>[2x]DTLESIDNCAVGCPTGGSSNVSIVRHAYTLNNNSTTKFANW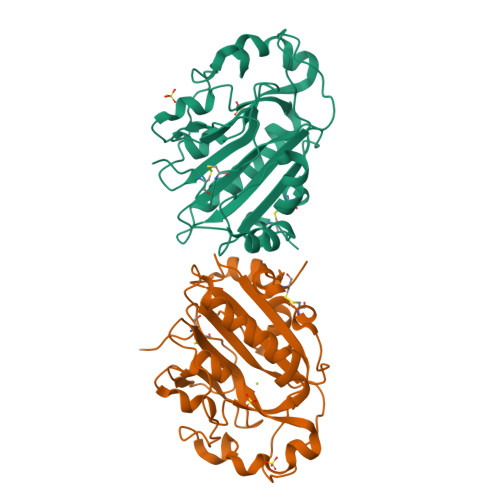VAYHITKDTPASGKTRNWKTDPALNPADTLAPADYTGANAALKVDRGHQAPLASLAGVSDWESLNYLSNITPQKSDLNQGAWARLEDQERKLIDRADISSVYTVTGPLYERDMGKLPGTQKAHTIPSAYWKVIFINNSPAVNHYAAFLFDQNTPKGADFCQFRVTVDEIEKRTGLIIWAGLPDDVQASLKSKPGVLPELMGCKN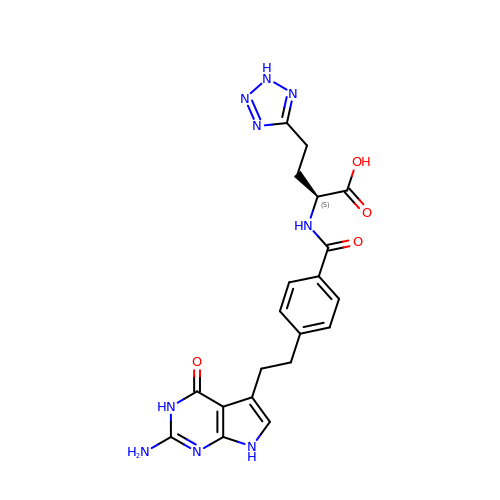2-{4-[2-(2-AMINO-4-OXO-4,7-DIHYDRO-3H-PYRROLO[2,3-D]PYRIMIDIN-5-YL)-ETHYL]-BENZOYLAMINO}-4-(2H-TETRAZOL-5-YL)-BUTYRIC ACID | C20 H21 N9 O4 | MXAFDBCLWLMXSI-ZDUSSCGKSA-N>MALFGYARVSTSQQSLDIQVRALKDAGVKANRIFTDKASGSSSDRKGLDLLRMKVKEGDVILVKK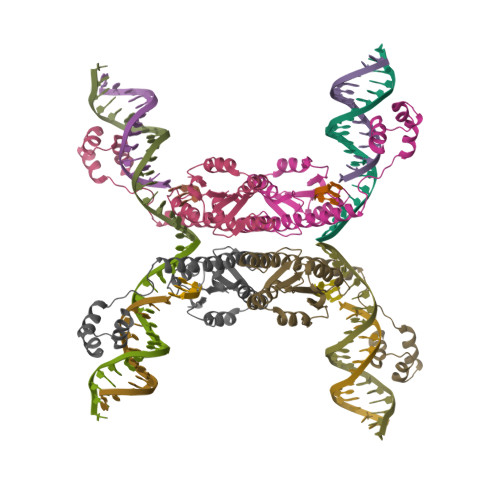LDRLGRDTADMIQLIKEFDAQGVSIRFIDDGISTDSYIGKMVVTILSAVAQAERQRILQRTNEGRQEAMAKGVVFGRKRKIDRDAVLNMWQQGLGASHISKTMNIARSTVYKVINESN[2x]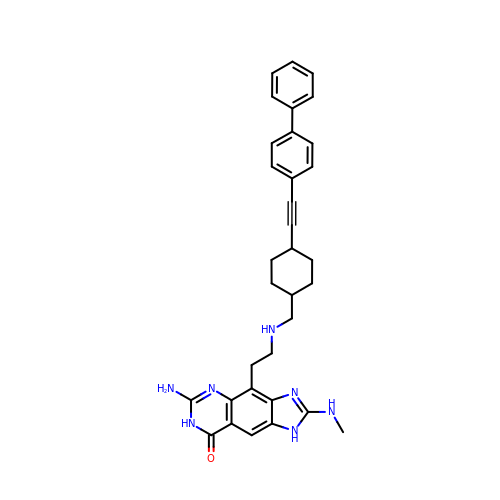6-amino-4-[2-({[trans-4-(biphenyl-4-ylethynyl)cyclohexyl]methyl}amino)ethyl]-2-(methylamino)-1,7-dihydro-8H-imidazo[4,5-g]quinazolin-8-one | C33 H35 N7 O | MEAOCIHCGKYHPF-AFARHQOCSA-N> SHSTAETTLDSFFSRAGLVGEIDLPLEGTTNPNGYANWDIDITGYAQMRRKVELFTYMRFDAEFTFVACTPTGQVVPQLLQYMFVPPGAPEPDSRESLAWQTATNPSVFVKLSDPPAQVSVPFMSPASAYQWFYDGYPTFGEHKQEKDLEYGACPNNMMGTFSVRTVGTSKSKYPLVIRIYMRMKHVRAWIPRPMRNQNYLFKANPNYAGNFIKPTGASRTAITT;> LTIGNSTITTQEAANIIVGYGEWPSYCSDSDATAVDKPTRPDVSVNRFYTLDTKLWEKSSKGWYWKFPDVLTETGVFGQNAQFHYLYRSGFCIHVQCNASKFHQGALLVAVLPEYVIGTVAGGTGTEDSHPPYKQTQPGADGFELQHPYVLDAGIPISQLTVCPHQWINLRTNNCATIIVPYINALPFDSALNHCNFGLLVVPISPLDYDQGATPVIPITITLAPMCSEFAGLRQ;> GFPTELKPGTNQFLTTDDGVSAPILPNFHPTPCIHIPGEVRNLLELCQVETILEVNNVPTNATSLMERLRFPVSAQAGKGELCAVFRADPGRSGPWQS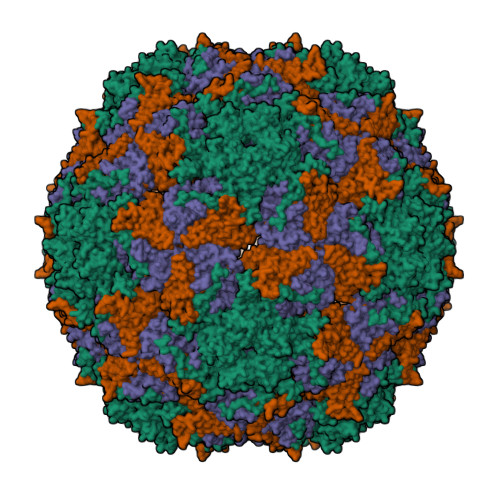TLLGQLCGYYTQWSGSLEVTFMFTGSFMATGKMLIAYTPPGGPLPKDRATAMLGTHVIWDFGLQSSVTLVIPWISNTHYRAHARDGVFDYYTTGLVSIWYQTNYVVPIGAPNTAYIIALAAAQKNFTMQLCKDASDIL> EFPEITEEMEKEIKNVFRNGNQDEVLSEAFRLTITRKDIQTLNHLNWLNDEIINFYMNMLMERSKEKGLPSVHAFNTFFFTKLKTAGYQAVKRWTKKVDVFSVDILLVPIHLGVHWCLAVVDFRKKNITYYDSMGGINNEACRILLQYLKQESIDKKRKEFDTNGWQLFSKKSQEIPQQMNGSDCGMFACKYADCITKDRPINFTQQH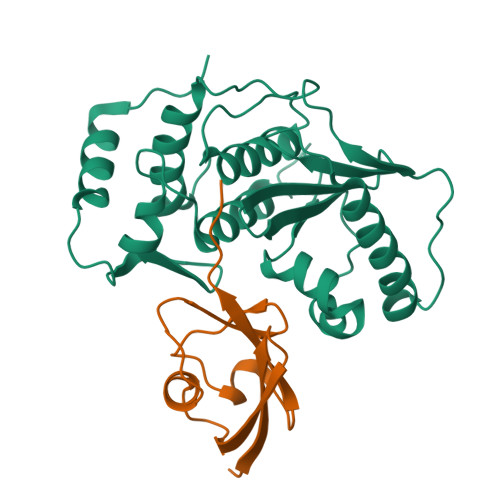MPYFRKRMVWEILHRKLL;> NDHINLKVAGQDGSVVQFKIKRHTPLSKLMKAYCERQGLSMRQIRFRFDGQPINETDTPAQLEMEDEDTIDVFQQQTGGVY(2E)-3-[7-(diethylamino)-2-oxo-2H-1-benzopyran-3-yl]prop-2-enal, bound form | C16 H19 N O2 | 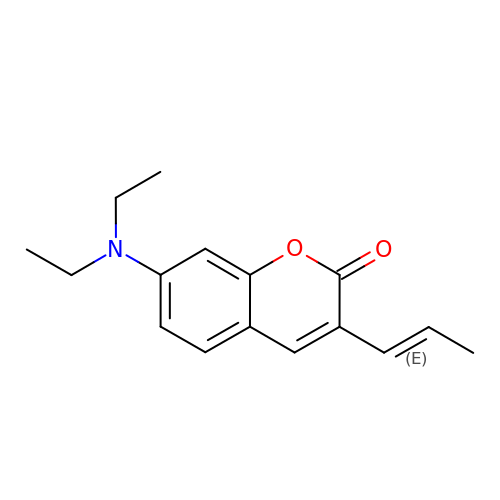YRIYSICZBXXPLJ-QPJJXVBHSA-N>[2x]MIVLFVDFDYFYAQVEEVLN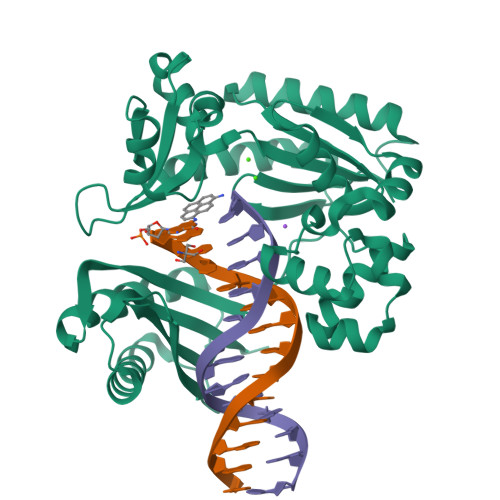PSLKGKPVVVCVFSGRFEDSGAVATANYEARKFGVKAGIPIVEAKKILPNAVYLPMRKEVYQQVSSRIMNLLREYSEKIEIASIDEAYLDISDKVRDYREAYNLGLEIKNKILEKEKITVTVGISKNKVFAKIAADMAKPNGIKVIDDEEVKRLIRELDIADVPGIGNITAEKLKKLGINKLVDTLSIEFDKLKGMIGEAKAKYLISLARDEYNEPIRTRVRKSIGRIVTMKRNSRNLEEIKPYLFRAIEESYYKLDKRIPKAIHVVAVTEDLDIVSRGRTFPHGISKETAYSESVKLLQKILEEDERKIRRIGVRFSKFIEAIGLDKFFDT> KY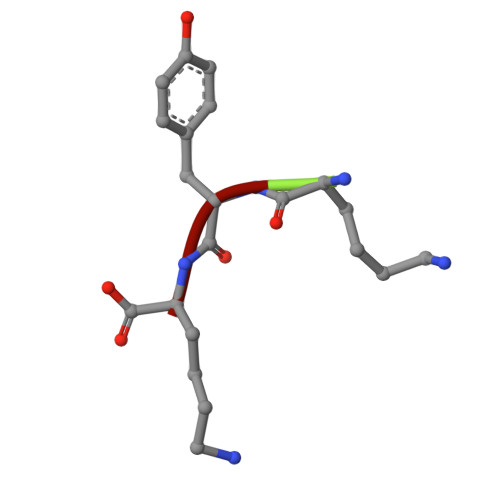K> MEGFKANLSLLRRPGEKTYTQRCRLFVGNLPADITEDEFKRLFAKYGEPGEVFINKGKGFGFIKLESRALAEIAKAELDDTPMRGRQLRVRFATHAAALSVRNLSPYVSNELLEEAFSQFGPIERAVVIVDDRGRSTGKGIVEFASKPAARKAF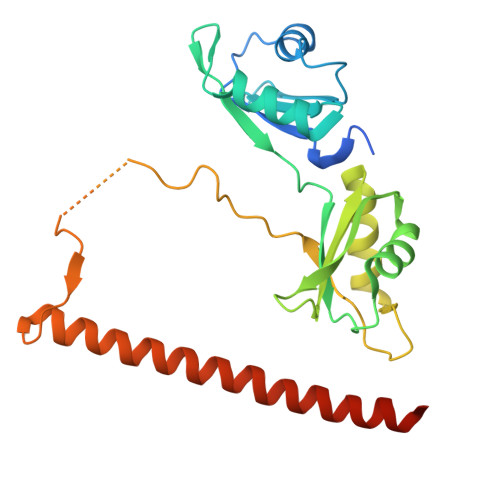ERCSEGVFLLTTTPRPVIVEPLEQLDDEDGLPEKLAQKNPMYQKERETPPRFAQHGTFEYEYSQRWKSLDEMEKQQREQVEKNMKDAKDKLESEMEDAYHEHQANLL4-methylpyridin-2-ol | C6 H7 N O | 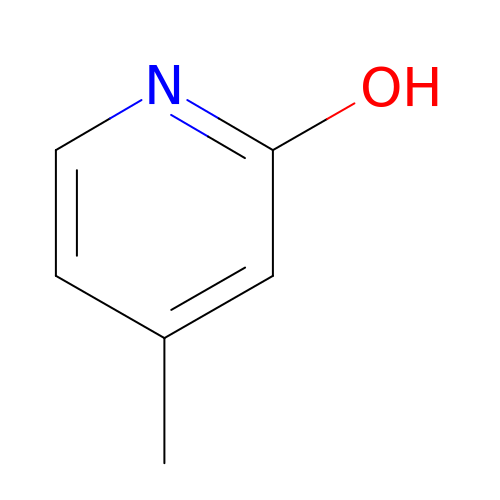YBDRFJXGJQULGH-UHFFFAOYSA-N>[6x]SRFESNPITLNDLSLGKPIAKGTNGVVYSAKVKDDETDDNKYPFALKMMFNYDIQENSMEILKAMYRETVPARMYYSNHDLNNWEIELANRRKHLPPHPNIVAIFSVFTDLYPAALPPRLHPEGEGRNMSLFLLMKRYDCNLQSFLSTAPSTRTSLLLLAQLLEGVAHMTAHGIAHRDLKSDNLLLDTSEPESPILVISDFGCCLADKTNGLSLPYTSYEMDKGGNTALMAPEIICQKPGTFSVLNYSKADLWAVGAIAYEIFNCHNPFYGPSRLKNFNYKEGDLPKLPDEVPTVIQALVANLLKRNPNKRLDPEVAANVCQLFLWAPSTWLKPGLKVPTSGEILQWLLSLTTKVLCEGKINNKSFGAAFTRNWRRTYPEYLLISSFLCRAKLANVRNALHWIQENLPELD

Autosomal recessive inherited loss-of-function mutations in human PTEN-induced kinase 1 (hPINK1), represent the second most frequent cause of early-onset Parkinson’s disease (PD). hPINK1 has been proposed to act as a master regulator of mitochondrial quality control, promoting the elimination of damaged mitochondria via autophagy known as mitophagy. In response to mitochondrial depolarisation, hPINK1 is activated and phosphorylates ubiquitin at Serine65 (Ser65). The molecular mechanisms of hPINK1 activation and substrate recognition are poorly understood. hPINK1 is distinct from other protein kinases due to the presence of three unique insertions (Ins1, Ins2 and Ins3) within the kinase domain and a C-terminal extension (CTE) of unknown function that bears no homology to any known protein domain. TcPINK1 exhibits constitutive catalytic activity towards ubiquitin, Parkin and generic substrates in vitro.

The crystal structure of a catalytically active fragment of TcPINK1 was solved and refined to 2.78 Å using E. coli expression of a cDNA construct encompassing the kinase domain and CTE (Ser150 - Asp570), and possessing mutations to reduce surface entropy (Glu527Ala and Lys528Ala), a 10 amino acid deletion in a large loop (Δ261–270), and a phospho-mimetic mutation (Ser205Glu). The N-lobe of the TcPINK1 kinase domain contains three insertions: Lys182–Pro192 (Ins1), Glu221–Ala253 (Ins2), and Leu260–Met288 (Ins3) and in contrast to hPINK1, Ins1 exists as a loop remnant in TcPINK1. Ins2 forms a small domain containing a βi-strand (222-226) and an αi-helix (231-242) followed by a loop (243-253). Ins3 is disordered and is not included in the final model. Finally, the majority of the TcPINK1 CTE (Ala487–Leu556) is α-helical in nature, and rather than forming a separate domain, is tightly packed on the E, G and H α-helices of the C-lobe of the kinase domain (3747 Å2 buried surface area), supporting previous data on the importance of this region for catalysis. Although TcPINK1 was crystallised without ATP, the kinase domain appears to adopt an active, closed conformation, based on the positioning of the αC helix, activation segment conformation, and the ‘in’ position of the DFG motif. Ser207 phosphorylation was also observed in the crystal structure. Inspection of the structure revealed that Glu205 (the phosphomimetic of Ser205) lies only 4 Å away from the tail (Asn287) of the disordered Ins3. Instead the TcPINK1 structure reveals that a highly conserved aspartate (Asp381) within the activation loop, an arginine residue (Arg336) of the HRD motif and an arginine residue (Arg216) in the αC-helix, form an equivalent interaction, which is further stabilized via interaction with basic residues (Lys212 on the αC-helix; Arg240 and Arg241 in Ins2) and another conserved aspartate (Asp366).(4~{S},6~{S})-4-[2,4-bis(fluoranyl)-5-pyrimidin-5-yl-phenyl]-6-(3,5-dimethyl-1,2-oxazol-4-yl)-4-methyl-5,6-dihydro-1,3-thiazin-2-amine 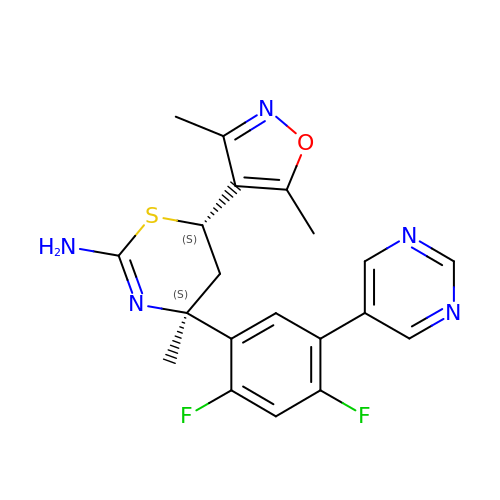| C20 H19 F2 N5 O S | UWUREBMKVJWTPP-PXNSSMCTSA-N>MADLAESNIKVMCRFRPLNESEVNRGDKYIAKFQGEDTVVIASKPYAFDRVFQSSTSQEQVYNDAAKKIVKDVLEGYNGTIFAYGQTSSGKVHTMEGKLHDPEGMGIIPRIVQDIFNYIYSMDENLEFHIKVSYFEIYLDKIRDLLDVSKTNLSVHEDKNRVPYVKGATERFVSSPDEVMDTIDEGKSNRHVAVTNMNEHSSRSHSIFLINVKQENTQTEQKLSGKLYLVDLAGSEKVSKTGAEGAVLDEAKNINKSLSALGNVISALAEGSTYVPYRDSKMTRILQDSLGGNARTTIVICCSPSSYNESETKSTLLFGQRAKTI[2x]

Kinesins are a family of microtubule-based motors that play important roles in intracellular transport and cell division. Kinesin-1 transports cargo within cells, a process tightly coupled with ATP hydrolysis. Whereas kinesin-1 in solution is mostly loaded with ADP, ADP release is accelerated several thousand-fold upon microtubule binding. Here we characterized kinesin-1 P-loop mutations that interfere with ADP binding and determined the structure of the corresponding mutated nucleotide-free kinesins.

We also found that when T92 is mutated to a valine, the nucleotide content of this mutant was very low compared with that of wild-type kinesin. Together with the observation that the T92V fluorescence does not increase upon incubation with mant-ADP, these data indicate that T92V has lost most of the kinesin affinity for ADP. We first determined the 2.0 Å resolution structure of T92V in a P21 space group crystal form. There were two similar molecules in the asymmetric unit, with a root mean square deviation (r.m.s.d.) after superposition of 0.47 Å (305 Cαs compared). The main difference between T92V and wild-type ADP-kinesin is the missing nucleotide and magnesium ion in the T92V nucleotide binding cleft. Instead of the nucleotide, an electron density, well accounted for by a sulfate ion that likely comes from the crystallization solution, is located close to the missing ADP β phosphate. However, in apo-T92V, helix α4, which is C-terminal to L11, starts at residue D249 instead of residue K256 in ADP-kinesin-1, i.e. is two turns longer. Finally, whereas T92 interacts with D231 in wild-type ADP-kinesin-1, this hydrogen bond is not formed in the T92V mutant, as expected. Therefore, we conclude from these observations that the T92V mutation disables Mg2+ binding, which would normally stabilize the ADP association and limit its release, and leads to a nucleotide-free kinesin without the need of an overall structural change towards the tubulin-bound apo-kinesin conformation. Therefore, an ADP-kinesin-like conformation can be adopted both by nucleotide-free wild-type kinesin and by the T92V mutant.>MKLVWTLSSWDDYEFWQRTDARMVEKINDLIRNAKRTPFAGLGKPEPLKGDMAGYWSRRITAEHRFV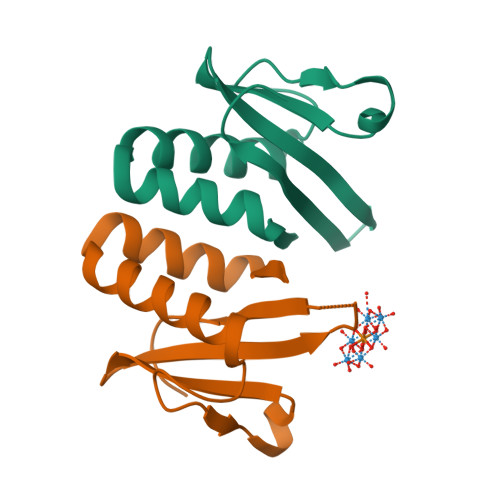YRVSGSGSEQRLEVIQCRFHYQLEVLFQ[2x]>GSKKWFSEFSIMWPGQAFSLKIKKILYETKSKYQNVLVFESTTYGKVLVLDGVIQLTEKDEFAYHEMMTHVPMTVSKEPKNVLVVGGG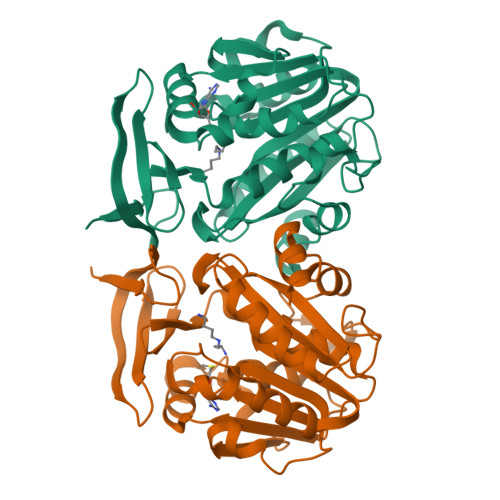DGGIIRELCKYKSVENIDICEIDETVIEVSKIYFKNISCGYEDKRVNVFIEDASKFLENVTNTYDVIIVDSSDPIGPAETLFNQNFYEKIYNALKPNGYCVAQCESLWIHVGTIKNMIGYAKKLFKKVEYANISIPTYPCGCIGILCCSKTDTGLTKPNKKLESKEFADLKYYNYENHSAAFKLPAFLLKEIENI[3x]> AA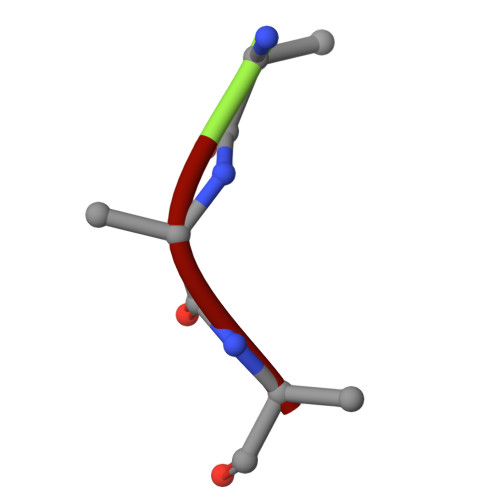A> EEEGRIRAMRAARSLGERTVTELILQHQNPQQLSSNLWAAVRARGCQFLGPAMQEEALKLVLLALEDGSALSRKVLVLFVVQRLEPRFPQASKTSIGHVVQLLYRASCFKVTKRDE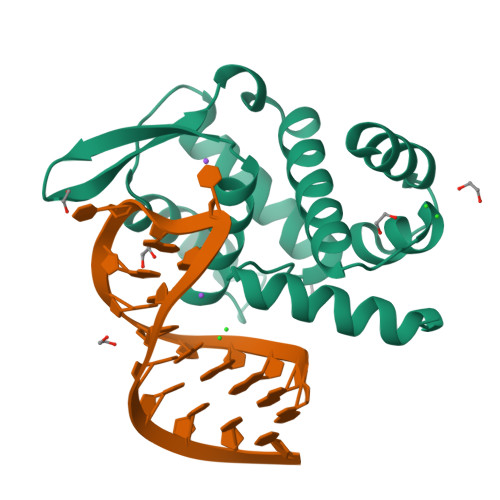DSSLMQLKEEFRTYEALRREHDSQIVQIAMEAGLRIAPDQWSSLLYGDQSHKSHMQSIIDKLQT> SMYVIRDEWGNQIWICPGCNKPD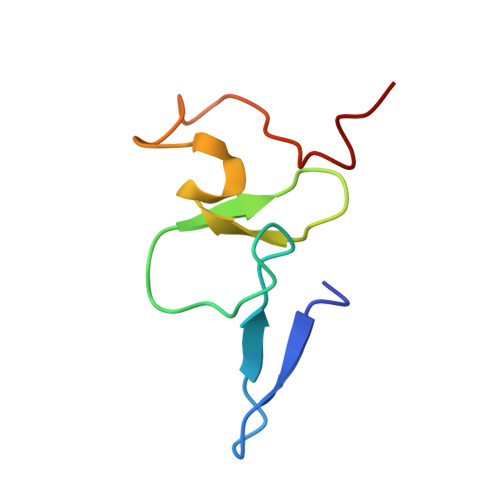DGSPMIGCDDCDDWYHWPCVGIMTAPPEEMQWFCPKCANK> MCTSVIYTAGDYYFGRNLDLEVNLGQEVVITPRNKTLEFREMPNLEHHYAIIGMSIVRDDYPLYFDGVNEKGVGMAGLNFDGPAHYFPVQEGKDNIASFELVPYILAAASSVAEAKKLLSN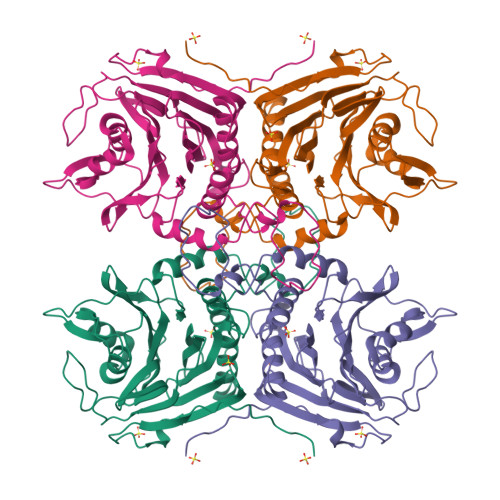ANIANINFSDKLQAAPLHWIIADKTGASVTVESTAKGLNVYDNPVGVLTNNPEFPRQLLNLSNYRSVAPANPANVFAPNVDLPVYSRGLGTHFLPGGMDSESRFVKATFTKMHAPVGNSEVENITNYFHILQSVEQQKGLDEVAPNTFEYTIYSDGSNLKKGIFYYKTYENSQINAVDMHKEDLEASELITYPVQNKQIINQQNHHHHHH> SNAHYQETQAVEAGEKTVEQFVQALNKGDYNKAAEMTSKKAANKSALSEKEILDKYQNIYGAADVKGLQISNLKVDKKDDSTYSFSYKAKMNTSLGELKDLSYKGTLDRNDGQTTINWQPNLVFPEMEGNDKVSLTTQEAARGNIIDRNGEPLATTGKLKQLGVVPSKLGDGGEKTANIKAIASSFDLTEDAINQAISQSWVQPDYFVPLKIIDGATPELPAGATIQEVDGRYYPLGEAAAQLIGYV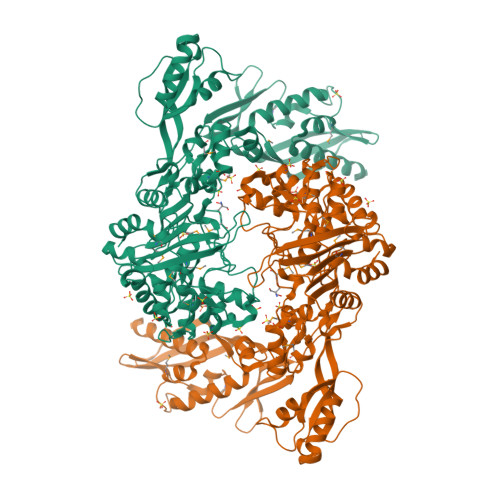GDITAEDIDKNPELSSNGKIGRSGLEMAFDKDLRGTTGGKLSITDADGVEKKVLIEHEVQNGKDIKLTIDAKAQKTAFDSLGGKAGSTVATTPKTGDLLALASSPSYDPNKMTNGISQEDYKAYEENPEQPFISRFATGYAPGSTFKMITAAIGLDNGTIDPNEVLTINGLKWQKDSSWGSYQVTRVSDVSQVDLKTALIYSDNIYMAQETLKMGEKKFRTGLDKFIFGEDLDLPISMNPAQISNEDSFNSDILLADTGYGQGELLINPIQQAAMYSVFANNGTLVYPKLIADKETKDKKNVIGETAVQTIVPDLREVVQDVNGTAHSLSALGIPLAAKTGTAEIKEKQDEKGKENSFLFAFNPDNQGYMMVSMLENKEDDDSATKRASELLQYLNQNYQ> RIALYIGNLTWWTTDEDLTEAVHSLGVNDI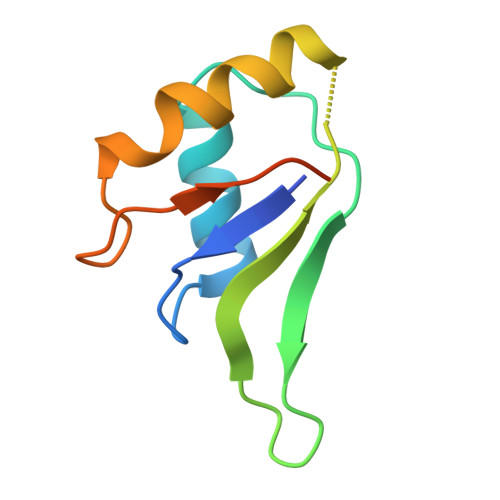LEIKFFENRANGQSKGFALVGVGSEASSKKLMDLLPKRELHGQNPVVTPSNKLEHHHHHH4-[4-({[(2,4-DICHLOROBENZOYL)AMINO]CARBONYL}AMINO)-2,3-DIMETHYLPHENOXY]BUTANOIC 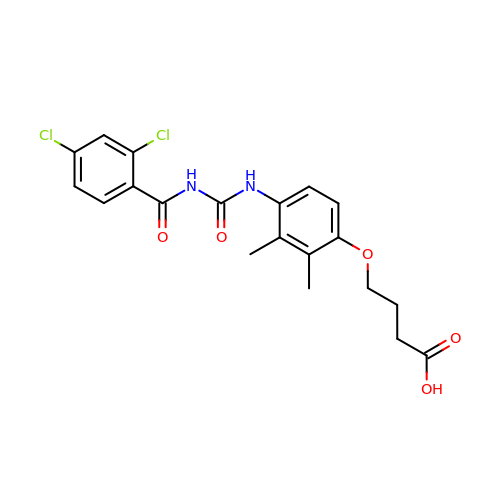ACID | C20 H20 Cl2 N2 O5 | FCEMCUPAYRPTLS-UHFFFAOYSA-N> MKSVFDIARSHVTFPVSRDGTALRRVLKDWLDYTECQSLQAKPAFPAELCITVHPSVKSMSRVYTQGDPKMSGEVCRRPGEAASLSYTKRVRLLLWSAVLPWEVQRGLSMSVLEPPGNGGSVLGEVGVRHGLGGSGGAVDGGSAVATKGWKEVEDSLGVVTDPTTXTAADFVSGPQCSTLGASIIPGMLFVMSPESAAQGLCFWSGAIRQPIDIAFIAPVEPPAADTPSFSELRQ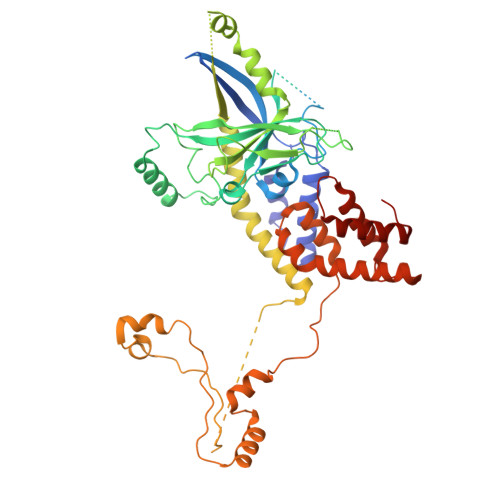RRLQLSLEGYDISRFFPDGELESPTVTFAVQSHSYLDPFPDCEQRDQQVGCGSSRERNKGIEDSRRYTATPEGVGRGNENVRYVLETRRNLLRDSIRSALRECRCTHGGVVWASNTGCAADGNPTGTGECDVEVTISLTLSDELKEDLREKARLYTNYVVPLEGHVRRHIKCLSGISPHPKGDATDGSDALQQKGTEAVWGEEGCVCTNGSAPFVAPPPIIKPPLPVKVGTLASTRPRSPMLADEAEGRPTRLAPSVFGRHDAPALQRAQQECNQLISASALARIPNTSPRAPEIPPIDYEIFDLCLRLGLCQSEAIYYFYGRIMREWSKELRRLRAAKSHGEGGVNDGNDMVLREEDVHRMLRLVHDPSLQVPPELSACVEAVASLRKITNEVGVPVV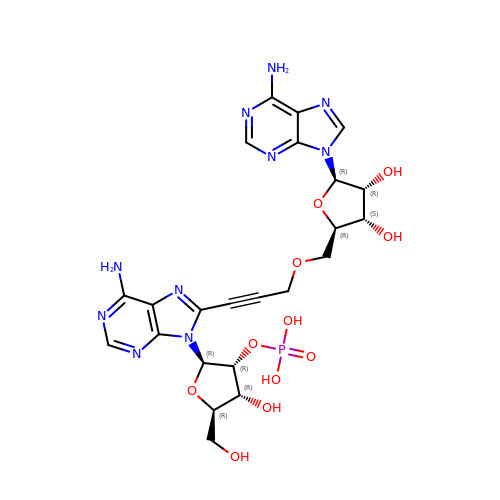[(2~{R},3~{R},4~{R},5~{R})-2-[8-[3-[[(2~{R},3~{S},4~{R},5~{R})-5-(6-aminopurin-9-yl)-3,4-bis(oxidanyl)oxolan-2-yl]methoxy]prop-1-ynyl]-6-azanyl-purin-9-yl]-5-(hydroxymethyl)-4-oxidanyl-oxolan-3-yl] dihydrogen phosphate | C23 H27 N10 O11 P | KWDXFYHXTKUVMJ-MKWZPUSRSA-N>[2x]DRHHHHHHKLGKMKIVEEPNSFGLNNPFLSQTNKLQPRVQPSPVSGPSHLFRLAGKCFNLVESTYKYELCPFHNVTQHEQTFRWNAYSGILGIWQEWDIENNTFSGMWMREGDSCGNKNRQTKVLLVCGKANKLSSVSEPSTCLYSLTFETPLVCHPHSLLVYPTLSEGLQEKWNEAEQALYDELITEQGHGKILKEIFRE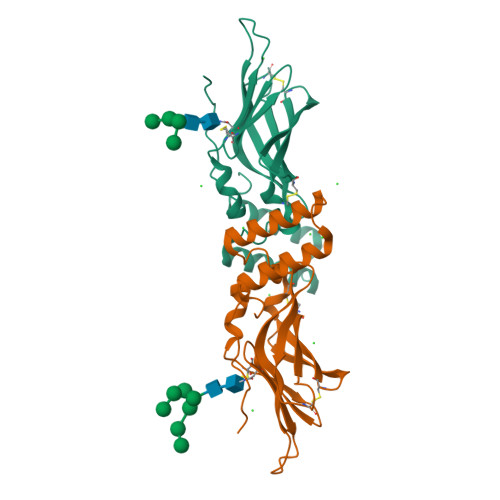AGYLKTTKPDGEGKETQDKPKEFDSLEKCNKGYTELTSEIQRLKKMLNEHGISYVTNGTSRSEGQPAEVNTTFARGEDKVHLRGDTGIRDGQ> KTSIVAS;>VPPAIVVLIGPPGYVGKQYPITASDIVIGRSVESQVYIDDKSLSRSHAKFAVNGSEVSVIDLGSTNKTIVNGQVIPPLA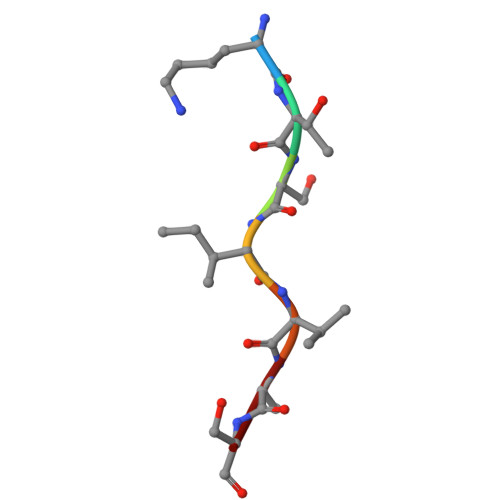SCLLKNNDQIKTGNVIFKFLEKGSIE[4x]> MDVLYSLSKTLKDARDKIVEGTLYSNVSDLIQQFNQMIITMNGNEFQTGGIGNLPIRNWNFDFGLLGTTLLNLDANYVETARNTIDYFVDFVDNVCMDEMVRESQRNGIAPQSDSLIKLSGIKFKRINFDNSSEYIENWNLQNRRQRTGFTFHKPNIFPYSASFTLNRSQPAHDNLMGTMWLNAGSEIQVAGFDYSCAINAPANTQQFEHIVQLRRVLTTATITLLPDAERFSFPRVITSADGATTWYFNPVILRPNNVEIEFLLNGQIINTYQARFGTIIARNFDTIRLS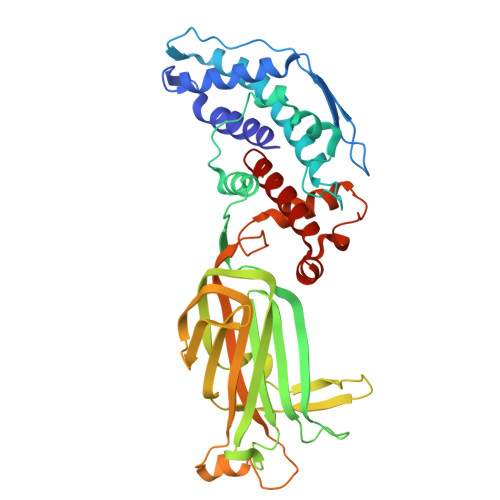FQLMRPPNMTPAVAALFPNAQPFEHHATVGLTLRIESAVCESVLADASETMLANVTSVRQEYAIPVGPVFPPGMNWTDLITNYSPSREDNLQRVFTVASIRSMLVK> MADKRA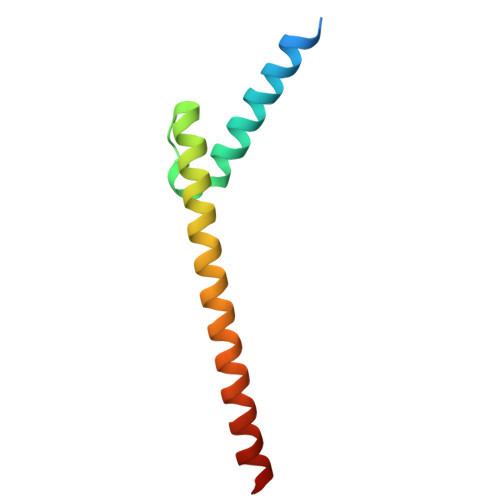HHNALERKRRDHIKDSFHSLRDSVPSLQGEKASRAQILDKATEYIQYMRRKNHTHQQDIDDLKRQNALLEQQVRALE> GTVLAEDQLAQMSKQLDMFKTNLEEFASKHKQEIRKNPEFRVQFQDMCATIGVDPLASGKGFWSEMLGVGDFYYELGVQIIEVCLALKHRNGGLITLEELH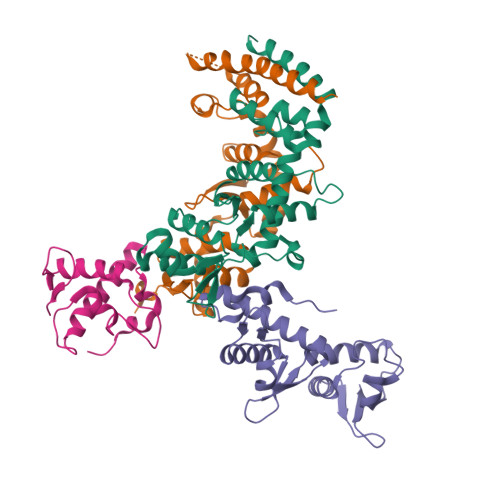QQVLKGRGKFAQDVSQDDLIRAIKKLKALGTGFGIIPVGGTYLIQSVPAELNMDHTVVLQLAEKNGYVTVSEIKASLKWETERARQVLEHLLKEGLAWLDLQAPGEAHYWLPALFTDLYSQEITAEEAREALP;> ETDKNISEAFEDLSKLMIKAKEMVELSKSIANKIKDKQGDITEDETIRFKSYLLSMGIANPVTRETYGSGTQYHMQLAKQLAGILQVPLEERGGIMSLTEVYCLVNRARGMELLSPEDLVNACKMLEALKLPLRLRVFDSGVMVIELQSHKEEEMVASALETVSEKGSLTSEEFAKLVGMSVLLAKERLLLAEKMGHLCRDDSVEGLRFYPNLFMTQS;>[2x]MAMSFEWPWQYRFPPFFTLQPNVDTRQKQLAAWCSLVLSFCRLHKQSSMTVMEAQESPLFNNVKLQRKLPVESIQIVLEELRKKGNLEWLDKSKSSFLIMWRRPEEWGKLIYQWVSRSGQNNSVFTLYELTNGEDTEDEEFHGLDEATLLRALQALQQEHKAEIITVSDGRGVKFF N-[3-(4-aminophenyl)propyl]adenosine 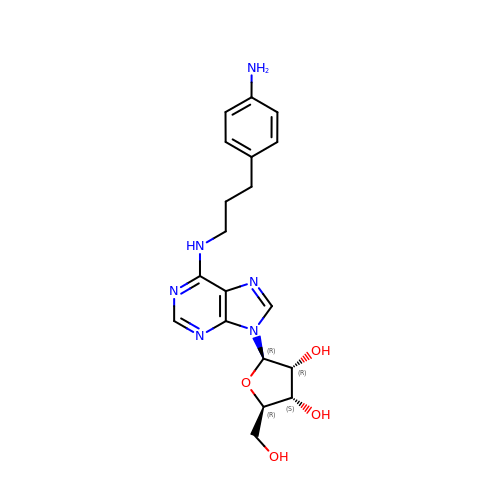| C19 H24 N6 O4 | ZGGQXDUSBXMHFX-NVQRDWNXSA-N2-chloro-N-(6-cyano-3-{2-[2-(2,4-dioxo-3,4-dihydropyrimidin-1(2H)-yl)ethoxy]phenoxy}-4-methylnaphthalen-1-yl)-N-methylacetamide | C27 H23 Cl N4 O5 | 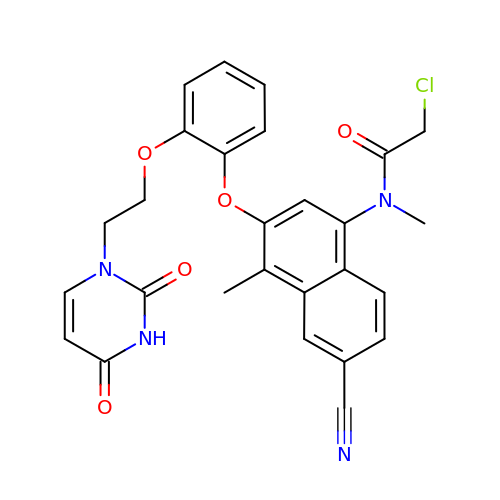MXVYCFLMSJUAJE-UHFFFAOYSA-N> GSDEKRLHFGNGHLKLPGLRTFVDPHTFEDPTQTVHEFAKELDATNISIDKVVGAGEFGEVCSGRLKLPSKKEISVAIKTLKVGYTEKQRRDFLGEASIMGQFDHPNIIRLEGVVTKSKPVMIVTEYMENGSLDSFLRKHDAQFTVIQLVGMLRGIASGMKYLSDMGYVHRDLAARNILINSNLVCKVSDFGLSRVLEDDPEAAYTTRGGKIPIRWTSPEAIAYRKFTSASDVWSYGIVLWEVMSYGERPYWEMSNQDVIKAVDEGYRLPPPMDCPAALYQLMLDCWQKDRNNRPKFEQIVSILDKLIRNPGSLKIITSAAARPSNLLLDQSNVDITTFRTTG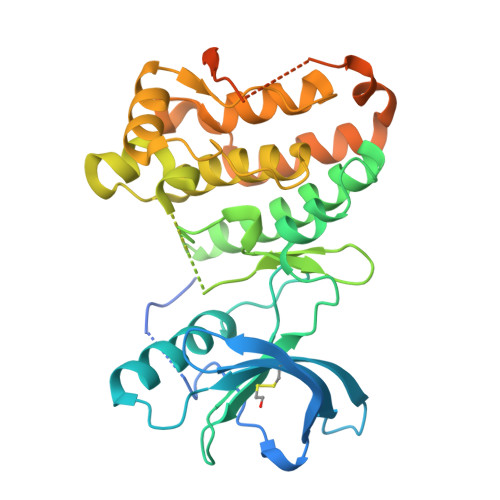DWLNGVWTAHCKEIFTGVEYSSCDTIAKIS>[8x]GSNAQAEEFKKY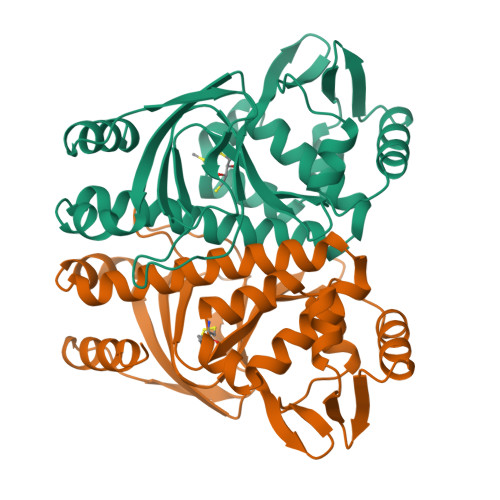LETNGIKPKQFHKKELIFNQWDPQEYCIFLYDGITKLTSISENGTIMNLQYYKGAFVIMSGFIDTETSVGYYNLEVISEQATAYVIKINELKELLSKNLTHFFYVFQTLQKQVSYSLAKFNDFSINGKLGSICSQLLILTYVYGKETPDGIKITLDNLTMQELGYSSGIAHSSAVSRIISKLKQEKVIVYKNSCFYVQNLDYLKRYAPKLDEWFYLACPATWGKLN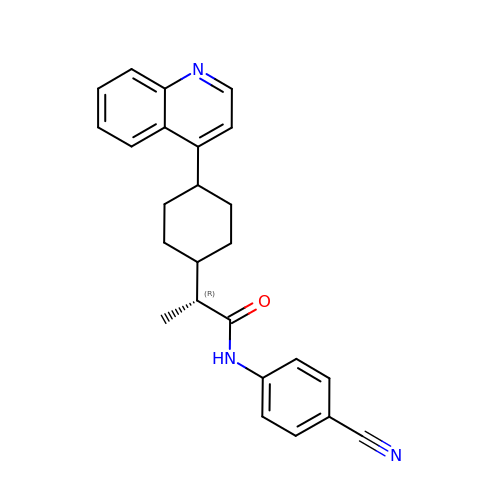(2R)-N-(4-cyanophenyl)-2-[cis-4-(quinolin-4-yl)cyclohexyl]propanamide | C25 H25 N3 O | GDSGPUWADCUKPY-RLLQIKCJSA-N8-AZAXANTHINE | C4 H3 N5 O2 | 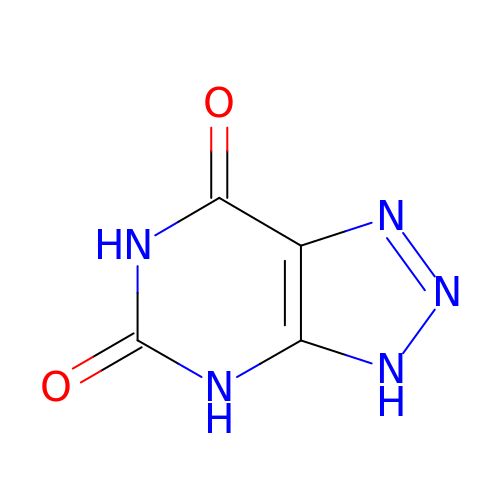KVGVQTOQSNJTJI-UHFFFAOYSA-N>GYALTEGEDYLVLDKPIPQEQSGKIEVLEFFGYFCVHCHHFDPLLLKLGKALPSDAYLRTEHVVWQPEMLGLARMAAAVN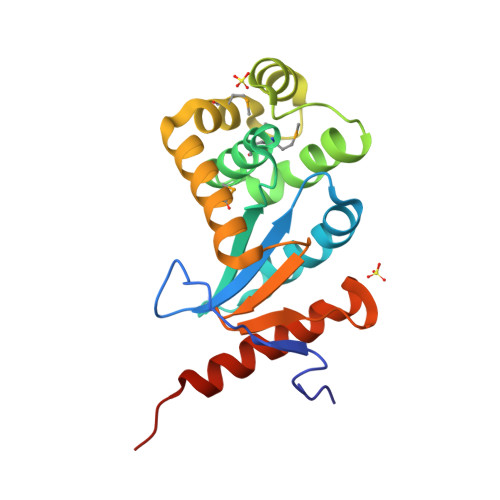LSGLKYQANPAVFKAVYEQKIRLENRSVAGKWALSQKGFDGKKLMRAYDSPEAAAAALKMQKLTEQYRIDSTPTVIVGGKYRVIFNNGFDGGVHTIKELVAKVREERKRQTPAVQK[2x]As the first reported host of “non-pathogenic-derived” pili, Lactobacillus rhamnosus GG is a gut-adapted commensal lactic acid bacterium (LAB) and one of many clinically investigated probiotic strains for human use in the prevention and treatment of certain gastric ailments. As with other Gram-positive bacteria, sortase-dependent piliation in L. rhamnosus GG (called SpaCBA) is assembled from the ~30 kDa SpaA (backbone), ~20 kDa SpaB (basal), and ~90 kDa SpaC (tip-located) pilins. Two immunoglobulin (Ig)-like subdomains comprise GG-SpaA, each having the conserved residues of a canonical E-box motif and internal isopeptide bonds formed between either lysine and asparagine or lysine and aspartate residues. Our findings show that the GG-SpaA structure has certain features in common with other pathogen-derived pilin-proteins, such as the Ig-like CnaB-type folds and the presence of internal isopeptide bonds6940.

As an alternative, GG-SpaA protein was fragmented by limited proteolysis as had been done previously for other backbone pilins. This produced a 15 kDa-sized fragment that can be crystallized in two different forms. The structure of the 15 kDa fragment was solved by the single anomalous dispersion method (SAD) using an ytterbium (Yb) derivative of the orthorhombic crystal form. Intriguingly, six metal ions are associated with the C-domain when the structure was solved using orthorhombic crystals. Metal ions are primarily coordinated by aspartates, but glutamate, lysine, and water from asymmetric and symmetric molecules also seem to participate. In the lanthanide derivative obtained by co-crystallization for SAD phasing, these metal ion-binding sites are mostly occupied by ytterbium ions.

>[4x]TYERTFVKKDAETKEVLEGAGFKISNSDGKFLKLTDKDGQSVSIGEGFIDVLANNYRLTWVAESDATVFTSDKSGKFGLNGFADNTTTYTAVETNVPDGYDAAANTDFKADNSSSDILDAPSGILPLEHHHHHH Oxygen activation in all heme enzymes requires the formation of high oxidation states of iron, usually referred to as ferryl heme. Ferryl heme refers broadly to a highly oxidized form of the heme in which the iron is in an oxidation state that is either one equivalent (FeIV, known as Compound II) or two equivalents (formally FeV, known as Compound I) above the resting oxidation state (FeIII). Here, we report 1.06 Å and 1.50 Å crystal structures for Compound II intermediates in cytochrome c peroxidase (CcP) and ascorbate peroxidase (APX), collected using the X‐ray free electron laser at SACLA. The results indicate that the ferryl species is finely tuned across Compound I and Compound II species in closely related peroxidase enzymes.

We thus developed an anaerobic procedure for direct formation of Compound II in CcP (see Experimental). Single crystal spectrophotometry at 100 K on crystals of CcP that had been reduced with dithionite under anaerobic conditions, followed by anaerobic reaction with H2O2 (see Experimental), showed absorption peaks for Compound II (λ max=530, 560 nm) that reproduce those in solution above. The Fe−O bond length extracted from this XFEL structure of CcP Compound II is 1.76 Å (with an error estimate from SHELX of 0.013 Å). Nonetheless, in this structure the Nϵ atom of His52 shows no density for a hydrogen atom and the imidazole is therefore more likely to be neutral (not protonated). The density for the guanidinium group of Arg48 is flat with all the hydrogens in‐plane, which is as expected when Arg48 is positively charged (Arg48 is also observed as charged in the neutron structure of Compound I). There are several key points to note when comparing with Compound I. First, the hydrogen bond patterns to the ferryl are the same in CcP Compound I and II (i.e. hydrogen bonds to the Nϵ atoms on Arg48 and the Nϵ proton of Trp 51) and do not allow space for a OH species bonded to the ferryl. These hydrogen bonds to Arg48 and Trp51 appear to be “locked in”, as the same hydrogen bonding pattern is observed in the X‐ray structure of CcP Compound I and in the neutron structure, Figure 5 B. Since the neutron structure of Compound I in CcP conclusively identifies a FeIV=O species (from the absence of nuclear density for a OH species), then we therefore interpret this ferryl species in Compound II of CcP as also being unprotonated (i.e. a FeIV=O species). That said, the bond length of 1.76 Å in this CcP Compound II structure is measurably and (within error) longer than that for CcP Compound I (1.63 Å). By comparison no such flexibility in hydrogen bonding to the distal Arg is observed in CcP, as the active site hydrogen bond structure is “locked” in a fixed arrangement that does not change between Compounds I and II.

> MKPLVHVASVEKGRSYEDFQKVYNAIALKLREDDEYDNYIGYGPVLVRLAWHTSGTWDKHDNTGGSYGGTYRFKKEFNDPSNAGLQNGFKFLEPIHKEFPWISSGDLFSLGGVTAVQEMQGPKIPWRCGRVDTPEDTTPDNGRLPDADKDADYVRTFFQRLNMNDREVVALMGAHALGKTHLKNSGYEGPWGAANNVFTNEFYLNLLNEDWKLEKNDANNEQWDSKSGYMMLPTDYSLIQDPKYLSIVKEYANDQDKFFKDFSKAFEKLLENGITFPKDAPSPFIFKTLEEQGL>MIQSQINRNIRLDLADAILLSKAKKDLSFAEIADGTGLAEAFVTAALLGQQALPADAARLVGAKLDLDEDSILLLQMIPLRGCIDDRIPTDP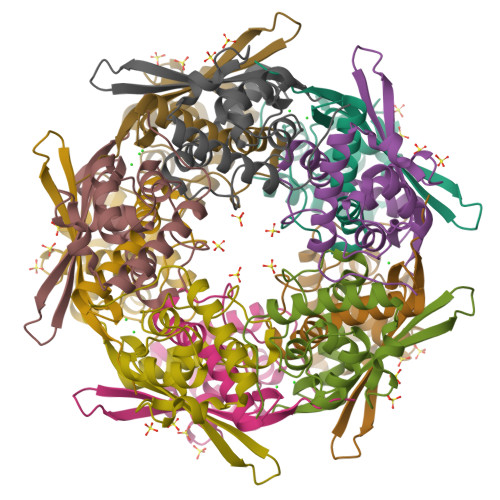TMYKFYEMLQVYGTTLKALVHEKFGDGIISAINFKLDVKKVADPEGGERAVITLDGKYLPTKPF[10x]>[4x]AAATTT

Previous studies by our group and by others have shown that bis(2-aminoimidazoline) drugs of this class are DNA minor groove binders with excellent affinity and selectivity toward AT-rich DNA regions. Here, we report a detailed study of the interaction of two new drugs, the bis(2-aminoimidazolinium) compounds 1 and 2, with AT-rich DNA sequences. Since kinetoplast DNA has a high content of AT-rich sequences, we aimed to discover whether parasite DNA was a target for these compounds inside the cell. Altogether, these results show that the N-phenylbenzamide bis(2-aminoimidazolinium) compounds 1 and 2 share the same mechanism of action against Trypanosoma brucei, acting specifically on the integrity of the kinetoplast by altering the structure and replication of kDNA.

Compound 2, a chloro analogue closely related to 1, was recently shown to be more potent than 1in vitro. In order to analyse the interactions of the chloro derivative 2 with DNA in our solved crystal structure, the hydrogen atom in ortho to the right-hand imidazoline ring was replaced with a chlorine atom. The compound 2 could adopt the equivalent place as compound 1 in the minor groove of the DNA duplex. Unexpectedly, the position of the chlorine atom in compound 2 prevents the interaction with the neighbouring DNA molecules, and therefore, the crystal packing would probably change to a C2 space group. Compounds 1 and 2 bound selectively to AT-containing DNA versus CG-containing DNA (from >10-fold to >60-fold). We found that compound 2 is able to displace HMGB1 (and also HMGA1a) proteins from their DNA binding sites. However, a 5-fold higher dosage (4 × 20 mg/kg/day i.p.) provided a 100% cure rate in this mouse model of stage 1 HAT.>PEIITPIITPFTKDNRIDKEKLKIHAENLIRKGIDKLFVNGTTGLGPSLS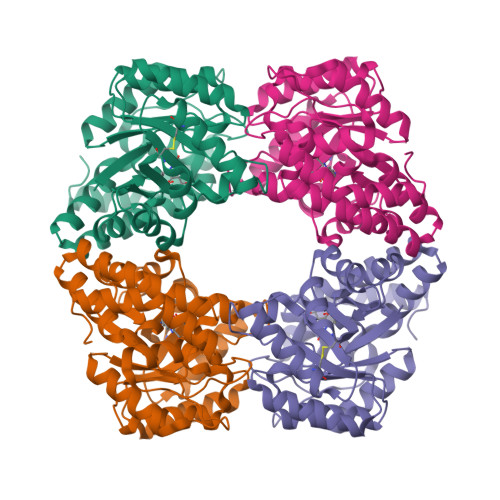PEEKLENLKAVYDVTNKIIFQVGGLNLDDAIRLAKLSKDFDIVGIASYAPYYYPRMSEKHLVKYFKTLCEVSPHPVYLYNYPTATGKDIDAKVAKEIGCFTGVKDVIENIIHTLDYKRLNPNMLVYSGSDMLIATVASTGLDGNVALGSNYLPEVTVTIKKLAMERKIDEALKLQFLHDEVIEASRIFGSLSSNYVLTKYFQGYDLGYPRPPIFPLDDEEERQLIKKVEGIRAKLVELKILKE[2x]2-[6-azanyl-9-[(2R,3R,4S,5R)-5-[[(azanylidene-$l^{4}-azanylidene)amino]methyl]-3,4-bis(oxidanyl)oxolan-2-yl]purin-8-yl]sulfanyl-N-[[(2R,3S,4R,5R)-5-(6-azanyl-8-bromanyl-purin-9-yl)-3,4-bis(oxidanyl)oxolan-2-yl]methyl]ethanamide | C22 H25 Br N14 O7 S | 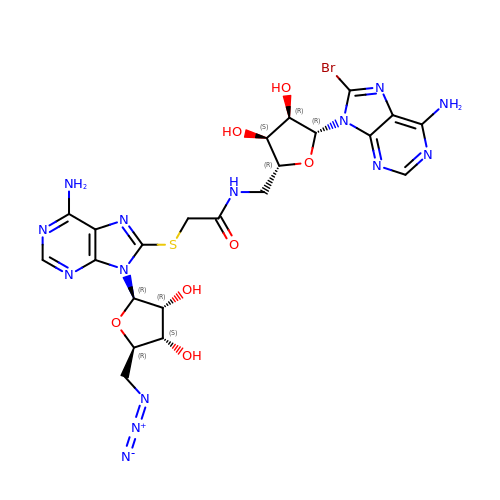WFFKQQMGOXMIGR-ZOUOOXKVSA-N(-)cis-chlordane | C10 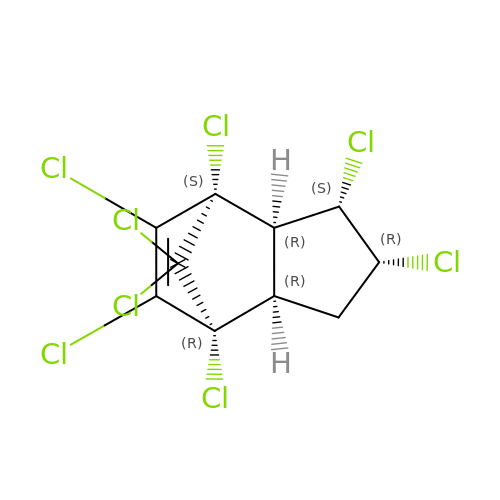H6 Cl8 | BIWJNBZANLAXMG-ISYKBROGSA-N>QAEILRAYARILEAQ[1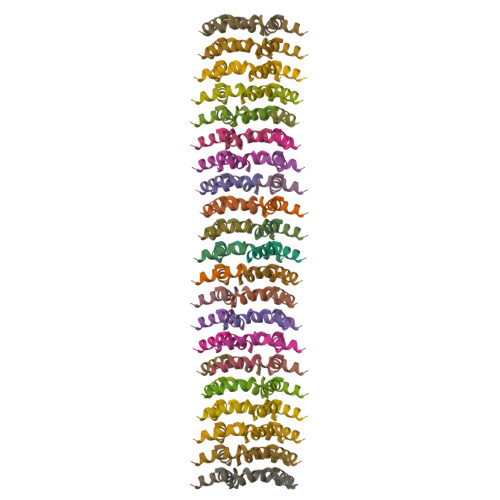05x]The most widespread dedicated NO sensor regulator in bacteria is NsrR, a member of the Rrf2 superfamily of homodimeric transcriptional regulators. NsrR proteins from Bacillus subtilis (Bs) and Streptomyces coelicolor (Sc) have been shown to bind a [4Fe–4S] cluster, which functions as the NO sensing module34. In ScNsrR, reaction with NO was shown to result in loss of the iron–sulfur (Fe–S) cluster and formation of iron-nitrosyl species. This process led to loss of high affinity DNA-binding and activation of genes that were previously repressed by [4Fe–4S] (holo-)ScNsrR, including those encoding Hmp-type NO detoxifying enzymes.

We also present the structure of a three-Cys-to-Ala (3CA) apo ScNsrR variant at 3.9 Å resolution. In spite of these limitations and because there were five ScNsrR monomers per asymmetric unit, we were able to solve its structure thereby gaining precious information about cluster-dependent DNA-binding modulation. Indeed, a comparison of the structures of wild-type holo and 3CA apo-ScNsrR shows that the [4Fe–4S] cluster conditions the conformation of two relevant regions. One of them is the C93EGDNPC99 sequence that forms a well-defined turn in the holo structure, but is less ordered in the apo structure where it adopts a different conformation; based on the superposition of the holo structure with that of the apo-IscR-DNA complex, the tip of this turn should contact the DNA backbone of the ScNsrR-binding site. Furthermore, Asn97 from the C93EGDNPC99 turn forms a H-bond with the carbonyl oxygen of Gly37, a residue situated in a turn next to the N terminus of the DNA recognition helix (RH). In the apo structure this interaction is no longer possible. In the apo structure the salt bridge between Asp8 and Arg12 appears to be preserved but the absence of the cluster changes the orientation of these residues causing the break of the H-bond between Arg12 and the carbonyl oxygen of Val36. The disruption of the Asn97-Gly37 and Arg12-Val36 H-bonds in apo-ScNsrR, indicated by the different conformation of the main chain in the medium-resolution apo structure, results in the displacement of the RH by over 2 Å, which may be enough to prevent its binding to DNA, as observed. The 3CA-ScNsrR apo structure shows that the conformation of the C93EGDNPC99 loop depends on the presence or absence of the Fe–S cluster. The other major determinant of the α3 RH orientation is Arg12 which, along with Asp8, significantly changes its position after cluster loss.

>MRLTKFTDLALRSLMRLAVVRDGDEPLATREVAEVVGVPYTHAAKAITRLQHLGVVEARRGRGGGLTLTDLGRRVSVGWLVRELEGEAEVVDAEGDNPAPLRGAARLRRALRDAQEAFYAALDPLTVTDLVAAPTGPVLLGLTDRPSGKLAAALEHHHHHH[5x]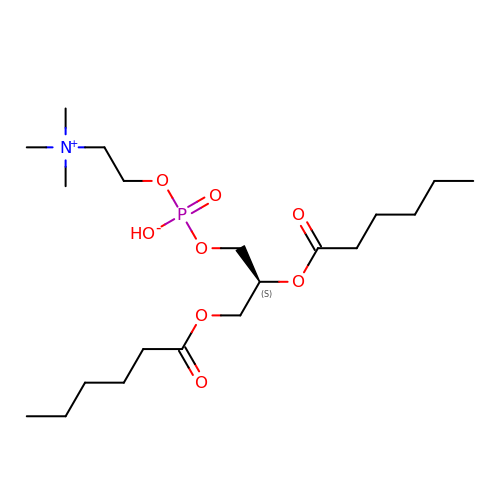(S)-2,3-bis(hexanoyloxy)propyl(2-(trimethylammonio)ethyl)phosphate | C20 H41 N O8 P | ZQODAMILHYQXDS-SFHVURJKSA-N>MKKKNVVVFGGGTGLSVLLRGLKTFPVSITAIVTVADDGGSSGRLRKELDIPPPGDVRNVLVALSEVEPLLEQLFQHRFENGNGLSGHSLGNLLLAGMTSITGDFARGISEMSKVLNVRGKVLPASNRSIILHGEMEDGTIVTGESSIPKAGKKIK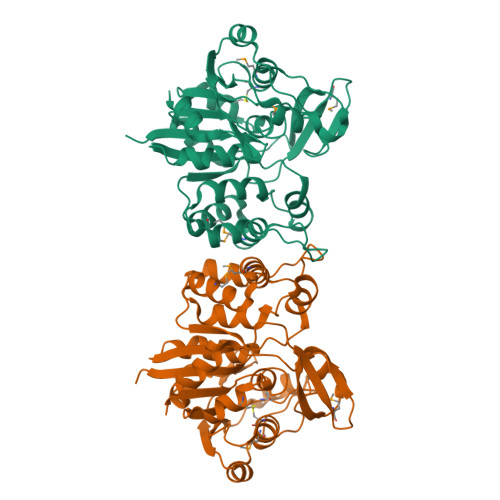RVFLTPKDTKPLREGLEAIRKADVIVIGPGSLYTSVLPNLLVPGICEAIKQSTARKVYICNVMTQNGETDGYTASDHLQAIMDHCGVGIVDDILVHGEPISDTVKAKYAKEKAEPVIVDEHKLKALGVGTISDYFVLEQDDVLRHNASKVSEAILEGKPRTSSSIQAAALEHHHHHH[4x]> EAKGLIRTWVTLKAEQTILPLVDEALQHTTTKGIVFQHPEIV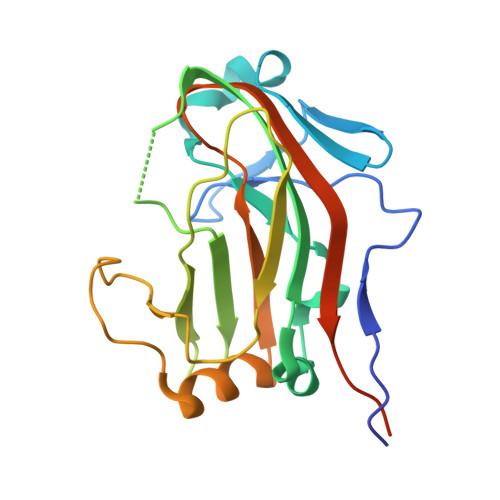AHMDLMREDLHLEPFYWKLPEQFEGKKLMAYGGKLKYAIYFEAREETGFSTYNPQVIIRGGTPTHARIIVRHMAAPLIGQLTRHEIEMTEKEWKYYGDDPRVHRTVTREDFLDILYDIHYILIKATYGNFMRQSRISEISMEVAEQGRGTTMTPPADLIEK hexadecyl dihydrogen phosphate | C16 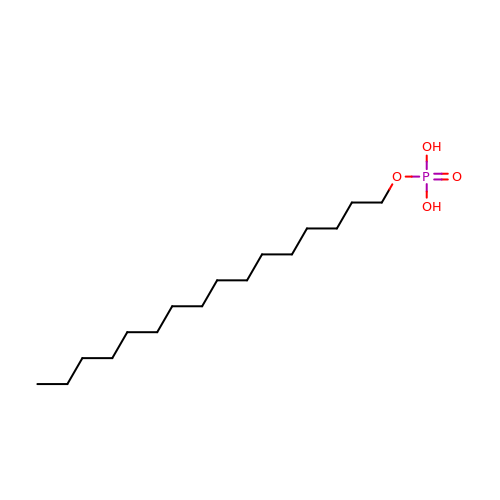H35 O4 P | ZUVCYFMOHFTGDM-UHFFFAOYSA-N Here we report on seven crystal structures of NP7 at low and high pH and with different heme ligands. The overall fold of NP7 resembles that of other NPs. Eight anti-parallel β-strands (A to H) form a barrel that hosts the heme cofactor including the ligation by the proximal His60 residue. One of the most interesting features of NP7 is its ability to bind to negatively charged membranes.

The analysis of the X-ray crystal structures of NP7 at low and high pH and with different heme ligands show the existence of a large resemblance in the overall fold, which is also similar to the spatial arrangement found in other NPs. These structures reveal the extensive clustering of Lys side-chains at the protein surface opposite the heme pocket, which is implicated in the charge-stabilized head-to-tail interaction observed in the crystal lattice. However, packing effects also explain the large structural similarity observed for the different ligand-bound and unbound structures, although such a structural similarity does not permit to rationalize the effect of deletion of the N-terminal residues on the binding affinities of certain ligands nor the pH sensitivity of NP7.

> LPGECSVNVIPKKNLDKAKFFSGTWYETHYLDMDPQATEKFCFSFAPRESGGTVKEALYHFNVDSKVSFYNTGTGPLESNGAKYTAKFNTVDKKGKEIKPADEKYSYTVTVIEAAKQSALIHICLQEDGKDIGDLYSVLNRNKNALPNKKIKKALNKVSLVLTKFVVTKDLDCKYDDKFLSSWQK;> GGG1-amino-4-hydroxy-9,10-dioxo-9,10-dihydroanthracene-2-carboxylic acid | C15 H9 N O5 | 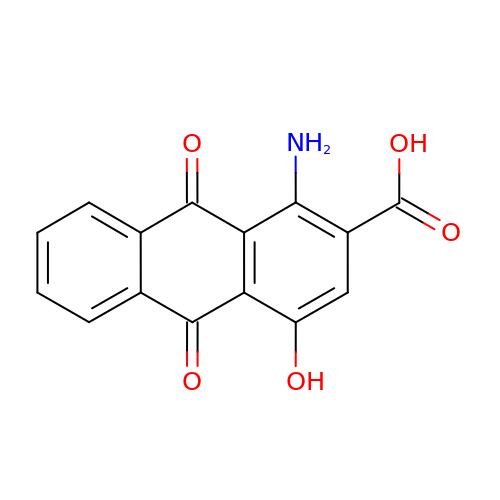MQFPVUCMBCTZAD-UHFFFAOYSA-N>METNLQKRKDSRKALRIK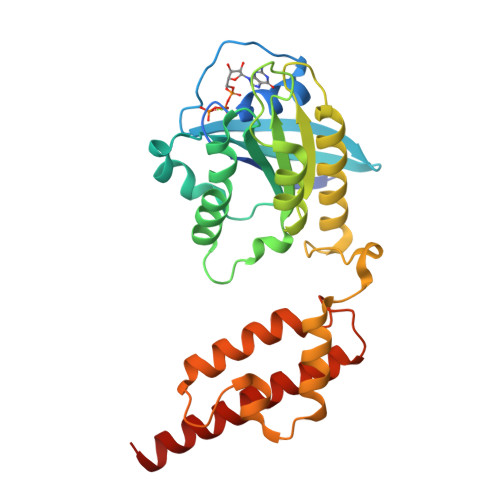VISMGNAEVGKSCIIKRYCEKRFVPKYQATIGIDYGVTKVHIKDREIKVNIFDMAGHPFFYEVRNEFYKDTQGVILVYDVGHKETFESLDGWLAEMKQELGPQGNIDNIVFAVCANKIDSTKHRSVDESEGRLWSESKGFLYFETSAQSGEGINEMFQAFYSAIVDLCDNGGKRPVSAINIGFTKEQADSIRRIRNCKDSWDMLGVKPGATRDEVNKAYRKLAVLLHPDKCMAPGSEDAFKAVVNARTALLKNIKLEHHHHHH[2x]> GPPGPPGPPGPKGHRGFSGLPGPPGP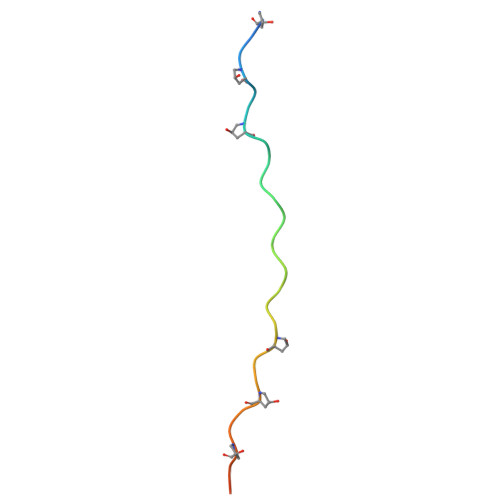PGPPGCCG>VANDENCGICRMAFNGCCPDCKVPGDDCP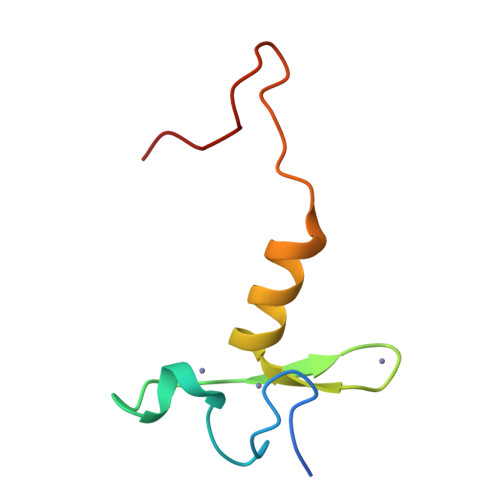LVWGQCSHCFHMHCILKWLHAQQVQQHCPMCRQEWKFKE[4x]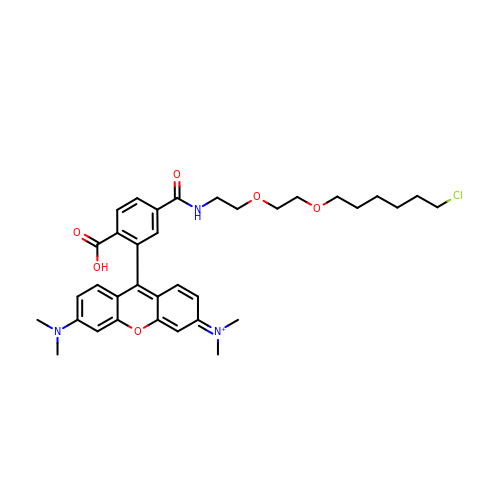[9-[2-carboxy-5-[2-[2-(6-chloranylhexoxy)ethoxy]ethylcarbamoyl]phenyl]-6-(dimethylamino)xanthen-3-ylidene]-dimethyl-azanium | C35 H43 Cl N3 O6 | YORHEDWUCXZZLS-UHFFFAOYSA-O>[2x]LEVQNSCDNCQPGTFCR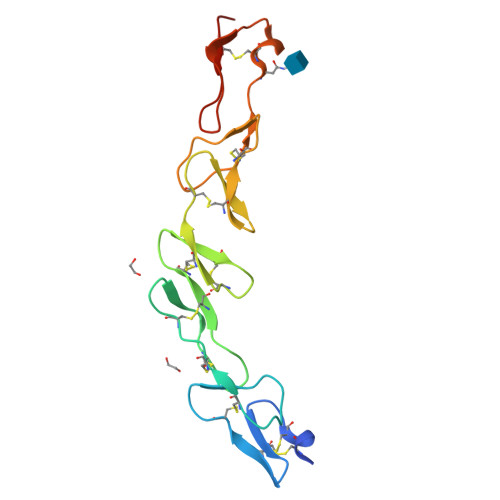KYNPVCKSCPPSTFSSIGGQPNCNICRVCAGYFRFKKFCSSTHNAECECIEGFHCLGPQCTRCEKDCRPGQELTKQGCKTCSLGTFNDQNGTGVCRPWTNCSLDGRSVLKTGTTEKDVVCGPLVPR> MKVTAAFAGLLVTAFAAPVPEPVLVSRSAGINYVQNYNGNLGDFTYDESAGTFSMYWEDGVSSDFVVGLGWTTGSSNAITYSAEYSASGSSSYLAVYGWVNYPQAE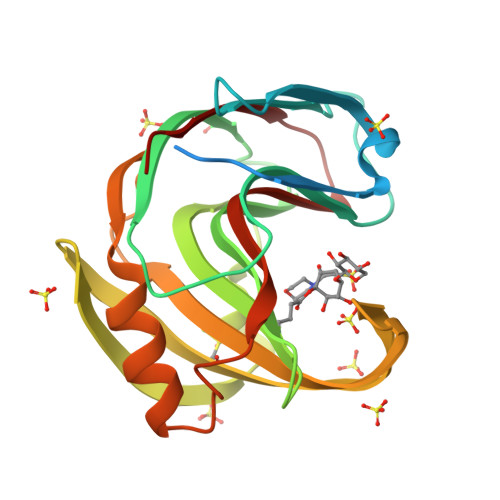YYIVEDYGDYNPCSSATSLGTVYSDGSTYQVCTDTRTNEPSITGTSTFTQYFSVRESTRTSGTVTVANHFNFWAQHGFGNSDFNYQVMAVEAWSGAGSASVTISS> AMADIGSEFGHRTLASTPALWASIPCPRSELRLDLVLPSGQSFRWREQSPAHWSGVLADQVWTLTQTEEQLHCTVYRGDKSQASRPTPDELEAVRKYFQLDVTLAQLYHHWGSVDSHFQEVAQKFQGVRLLRQDPIECLFSFICSSNNNIARITGMVERLCQAFGPRLIQLDDVTYHGFPSLQALAGPEVEAHLRKLGLGYRARYVSASARAILEEQGGLAWLQQLRESSYEEAHK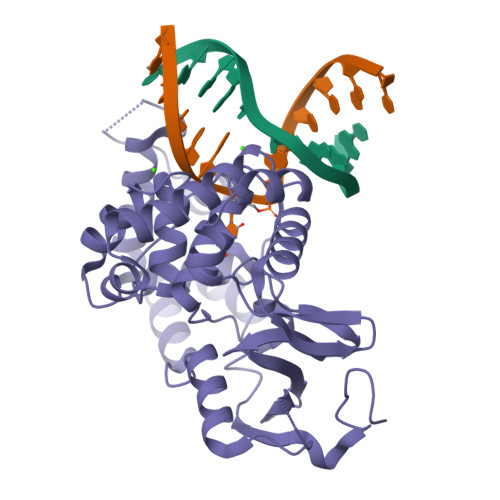ALCILPGVGTKVADCICLMALDKPQAVPVDVHMWHIAQRDYSWHPTTSQAKGPCPQTNKELGNFFRSLWGPYAGWAFAVLFSADLRQSR> MDNTILILGDXLSAAYGLQQEEGWVKLLQDKYDAEQSDIVLINASISGETSGGALRRLDALLEQYEPTHVLIELGANDGLRGFPVKKMQTNLTALVKKSQAANAMTALMEIYIPPNYGPRYSKMFTSSFTQISEDTNAHLMNFFMLDIA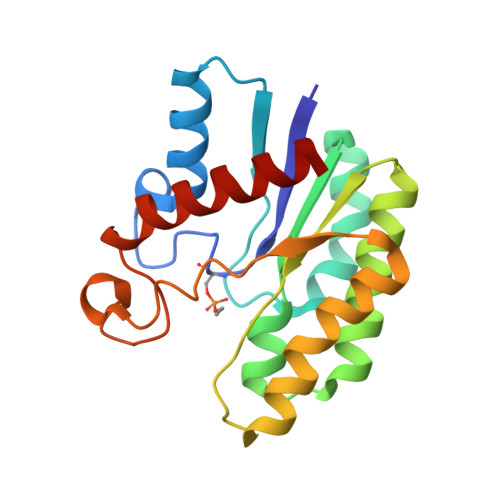GKSDLMQNDSLHPNKKAQPLIRDEMYDSIKKWLNNV> MHHHHHHSSRENLYFQGGSSEFQINEQVLACWSDCRFYPAKVTAVNKDGTYTVKFYDGVVQTVKHIHVKAFSKDQNIVGN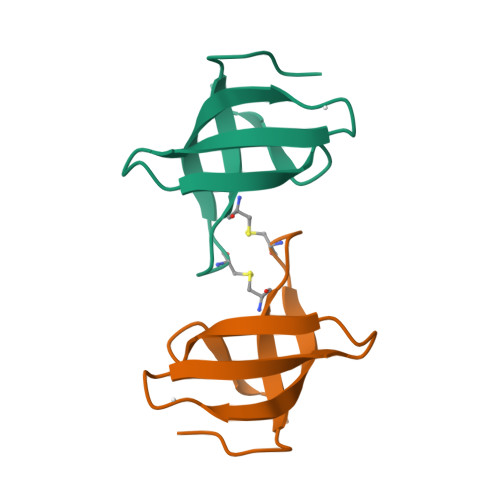ARPKE[(2~{R},3~{S},4~{S})-5-[(4~{a}~{R})-7,8-dimethyl-2,4-bis(oxidanylidene)-4~{a},5-dihydropyrimido[4,5-b]quinolin-10-yl]-2,3,4-tris(oxidanyl)pentyl] dihydrogen 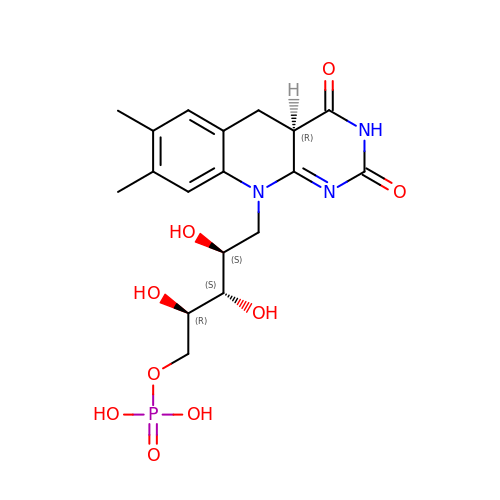phosphate | C18 H24 N3 O9 P | MPTDYDRCOLGCLP-BEAPCOKYSA-N> TVAYIAIGSNLASPLEQVNAALKALGDIPESHILTVSSFYRTPPLGPQDQPDYLNAAVALETSLAPEELLNHTQRIALQQGRVRKAERWGPRTLDLDIMLFGNEVINT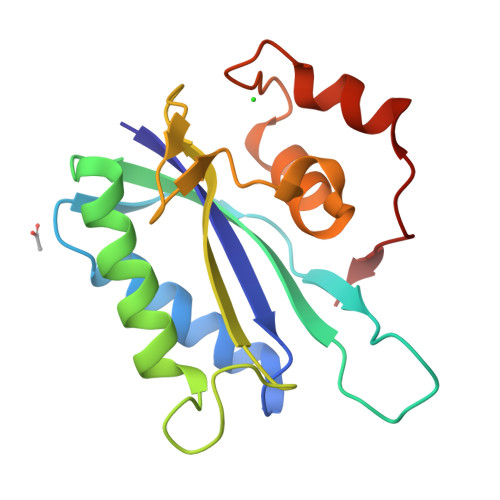ERLTVPHYDMKNRGFMLWPLFEIAPELVFPDGEMLRQILHTRAFDKLNKW>MIRYPNGKTFQPKHSVSSQNSQKRAPSYSNRGMTLEDDLNETNKYYLTNQIAVIHKKPTPVQIVNVHYPKRSAAVIKEAYFKQSSTTNYNGIYKGRYIDFEAKETKNKTSFPLQNFHDHQIEHMKQVKAQDGICFVIISAFDQVYFLEADKLFYFWDRKEKNGRKSIRKDELEETAYPISLGYAPRIDYISIIEQLYF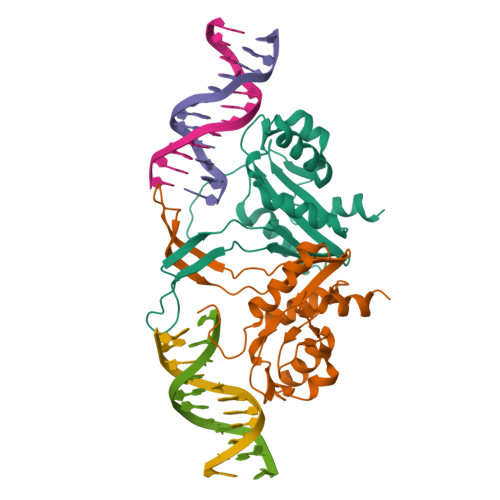S[4x]>[6x]MGHMNLTELKNTPVSELITLGENMGLENLARMRKQDIIFAILKQHAKSGEDIFGDGVLEILQDGFGFLRSADSSYLAGPDDIYVSPSQIRRFNLRTGDTISGKIRPPKEGERYFALLKVNEVNFDKPENARNKILFENLTPLHANSRLRMERGNGSTEDLTARV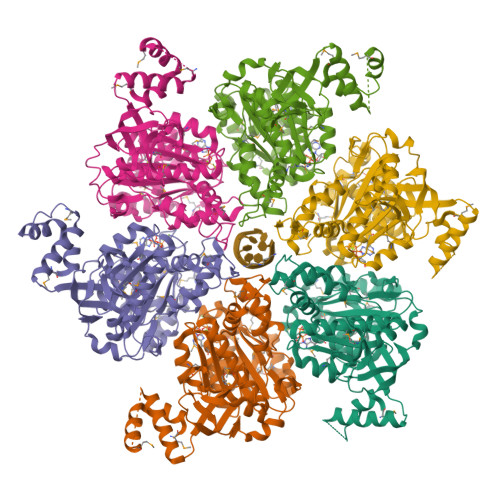LDLASPIGRGQRGLIVAPPKAGKTMLLQNIAQSIAYNHPDCVLMVLLIDERPEEVTEMQRLVKGEVVASTFDEPASRHVQVAEMVIEKAKRLVEHKKDVIILLDSITRLARAYNTVVPASGKVLTGGVDANALHRPKRFFGAARNVEEGGSLTIIATALIDTGSKMDEVIYEEFKGTGNMELHLSRKIAEKRVFPAIDYNRSGTRKEELLTTQEELQKMWILRKIIHPMGEIDAMEFLINKLAMTKTNDDFFEMMKRS>[2x]MVLYFIGMGLYDERDITVKGLEIAKKCDYVFAEFYTSLMAGTTLGRIQKLIGKEIRVLSREDVELNFENIVLPLAKENDVAFLTPGDPLVATTHAELRIRAKRAGVESYVIHAPSIYSAVGITGLHIYKFGKSATVAYPEGNWFPTSYYDVIKENAERGLHTL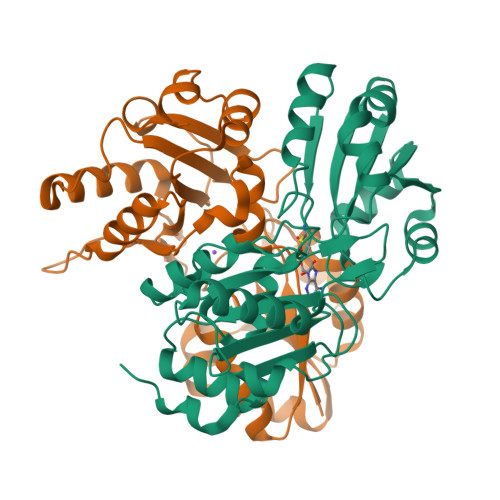LFLDIKAEKRMYMTANEAMELLLKVEDMKKGGVFTDDTLVVVLARAGSLNPTIRAGYVKDLIREDFGDPPHILIVPGKLHIVEAEYLVEIAGAPREILRVNV> GGSMASMDFPQHSQHVLEQLNQQRQLGLLCDCTF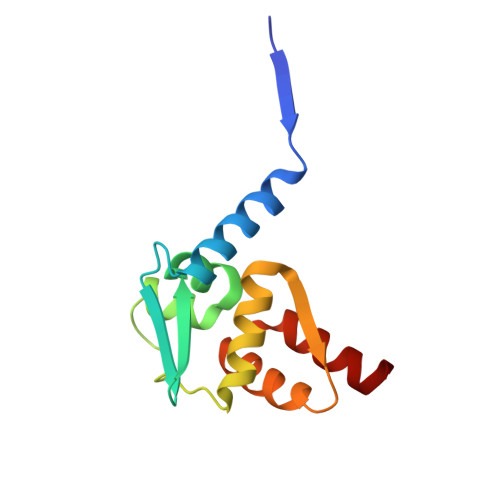VVDGVHFKAHKAVLAACSEYFKMLFVDQKDVVHLDISNAAGLGQVLEFMYTAKLSLSPENVDDVLAVATFLQMQDIITACHALKSLA>MCPTLNNIVSSLQRNGIFINSLIAALTIGGQQLFSSSTFSCPCQVGKNFYYGSAFLVIPALILLVAGFALRSQMWTITGEYCCSCAPPYRRISPLECKLACLRFFSITGRAVIAPLTWLAVTLLTGTYYECAASEFASVDHYPMFDNVSASKREEILAGFPCCRSAPSDVILVRDEIALLHRYQSQMLGWILITLATIAALVSCCVAKCCSPLTSLQHCYWTSHLQNERELFEQAAEQHSRLLMMHRIKKLFGFIPGSEDVKHIRIPSCQDWKDISVPTLLCMGDDLQGHYSFLGNRV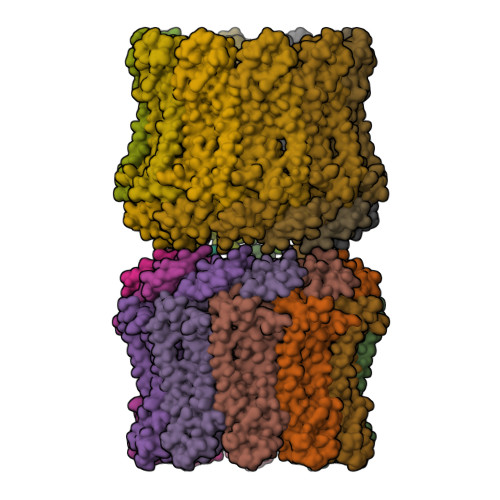DEDNEEDRSRGIELKP[20x]N6-(2,5-DIMETHOXY-BENZYL)-N6-METHYL-PYRIDO[2,3-D]PYRIMIDINE-2,4,6-TRIAMINE | 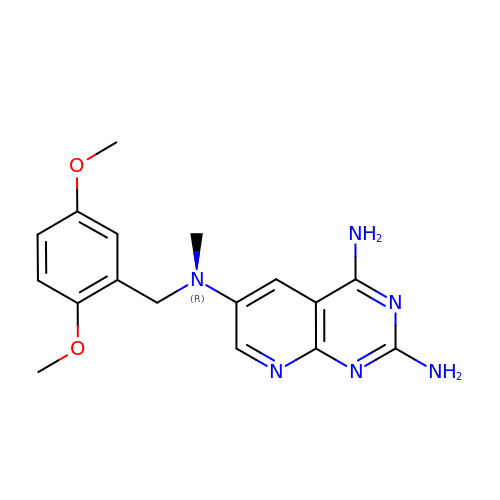C17 H20 N6 O2 | HZTFNSCZLJLPEO-UHFFFAOYSA-N PHOSPHONATE 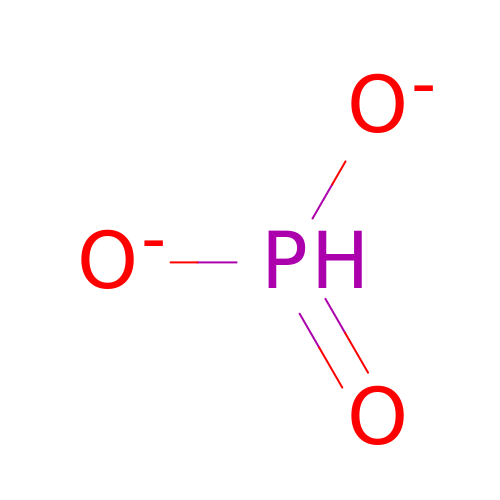| H O3 P | ABLZXFCXXLZCGV-UHFFFAOYSA-L> GKLSLQDVAELIRARACQRVVVMVGAGISTPSGIPDFRSPGSGLYSNLQQYDLPYPEAIFELPFFFHNPKPFFTLA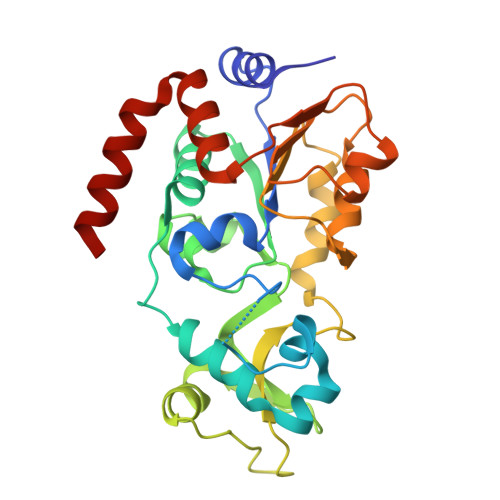KELYPGNYKPNVTHYFLRLLHDKGLLLRLYTQNIDGLERVSGIPASKLVEAHGTFASATCTVCQRPFPGEDIRADVMADRVPRCPVCTGVVKPDIVFFGEPLPQRFLLHVVDFPMADLLLILGTSLEVEPFASLTEAVRSSVPRLLINRDLVGPLAWHPRSRDVAQLGDVVHGVESLVELLGWTEEMRDLVQRETGKL>MAHHHHHHSAALEVLFQGPGSEDGPVTNPRQEEPQKVVKEEGFARGADVSWLTQME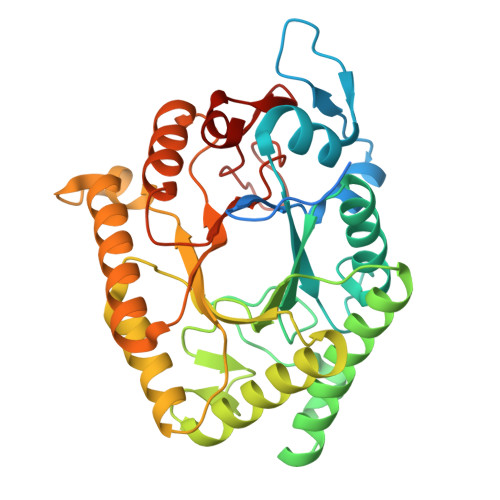AEGLKFYTPDENRQEMECMDLLRDYCGVNSIRLRVWVNPKDGWNNMNDVIVKAKRAERLGLRTMIDFHFSDTWADPGHQEMPEAWKELSFDDLKIALSEHVKSVLTALKAVGVTPEWVQVGNETTPGMMLPVGSVDNPEQLTALNNAGYDAVKAICPDAKVIVHLDAGNDQWVYNRMFDILQANGGKYDMIGMSLYPYWAEQEGKTGGWLKVADDCIANIKHVKQKYNKPVMICEIGMPYDQAEACKQLITKMMQADVEGIFYWEPQAPNGYNDGYNLGCFDNNAPTIALDAFKIQ[2x]>GHMALDEAPAEARPGSRAVELEIDGRSRIFDIDDPDLPKWIDEEAFRSDDYPYKKKLDREEYEETLTKLQIELVKVQFWMQATGKRVMAVFEGRDAAGKGGAIHATTANMNPRSARVVALTKPTETERGQWYFQRYVATFPTAGEFVLFDRSWYNRAGV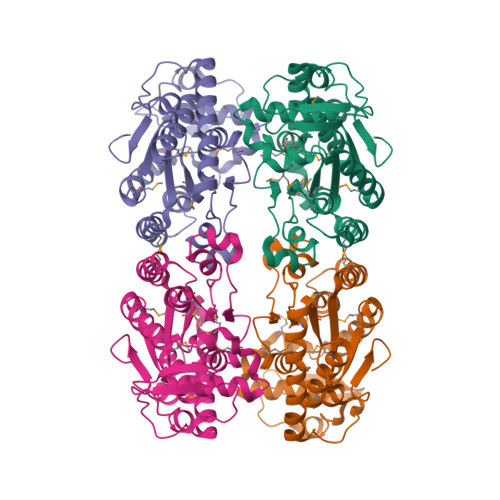EPVMGFCTPDQYEQFLKEAPRFEEMIANEGIHLFKFWINIGREMQLKRFHDRRHDPLKIWKLSPMDIAALSKWDDYTGKRDRMLKETHTEHGPWAVIRGNDKRRSRINVIRHMLTKLDYDGKDEAAIGEVDEKILGSGPGFLRGS[4x]>[16x]IKVGINGFGRIGRIVFRAAQKRSDIEIVAINDLLDADYMAYMLKYDSTHGRFDGTVEVKDGHLIVNGKKIRVTAERGPANLKWDEVGVDVVAEATGLFLTDETARKHITAGAKKVVMTGPSKDNTPMFVKGANFDKYAGQDIVSNASCTTNCLAPLAKVINDNFGIIEGLMTTVHATTATQKTVDGPSHKDWRGGRGASQNIIPSSTGAAKAVGKVLPELNGKLTGMAFRVPT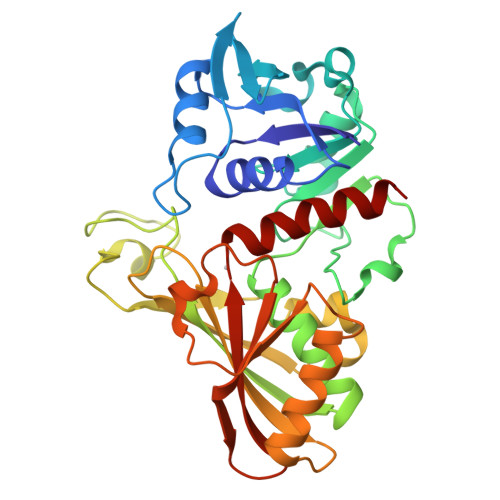PNVSVVDLTVRLEKAATYEQIKAAVKAAAEGEMKGVLGYTEDDVVSTDFNGEVCTSVFDAKAGIALNDNFVKLVSWYDNETGYSNKVLDLIAHISK>MAHCTEYMNAPKKLPADVAEELATTAQKLVQAGKGILAADESTQTIKKRFDNIKLENTIENRASYRDLLFGTKGLGKFISGAILFEETLFQKNEAGVP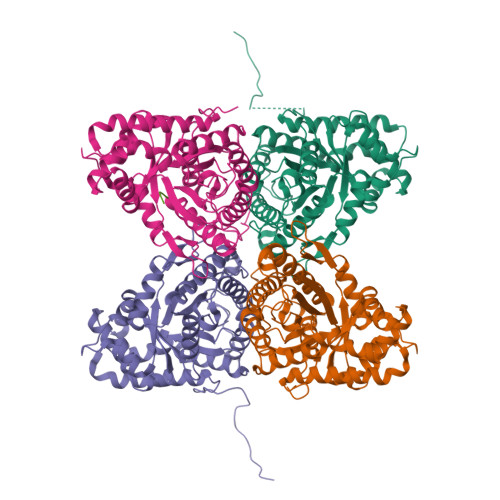MVNLLHNENIIPGIKVDKGLVNIPCTDEEKSTQGLDGLAERCKEYYKAGARFAKWRTVLVIDTAKGKPTDLSIHETAWGLARYASICQQNRLVPIVEPEILADGPHSIEVCAVVTQKVLSCVFKALQENGVLLEGALLKPNMVTAGYECTAKTTTQDVGFLTVRTLRRTVPPALPGVVFLSGGQSEEEASVNLNSINALGPHPWALTFSYGRALQASVLNTWQGKKENVAKAREVLLQRAEANSLATYGKYKGGAGGENAGASLYEKKYVY[4x];> EDNDWN>[4x]MKYVVVSGGVISGIGKGVLASSTGMLLKTLGLKVTSIKIDPYMNIDAGTMSPLEHGECFVLDDGGETDLDLGNYERYLGITLSRDHNITTGKIYSHVISRERRGDYLGKTVQIVPHLTNAIQDWIQRVSKIPVDDTGLEPDVCIIELGGTVGDIESAPFVEAL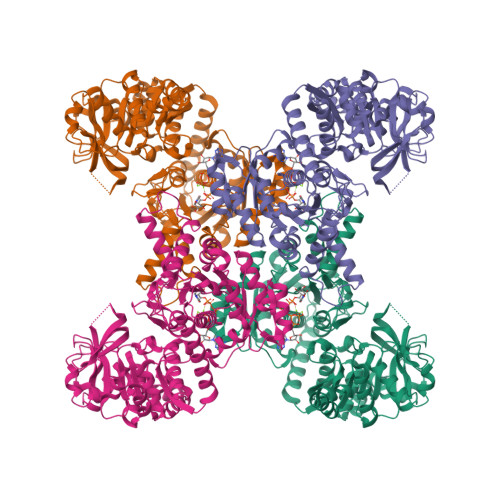RQFQFEVGRENFALIHVSLVPVIHGEQKTKPTQAAIKDLRSLGLIPDMIACRCSEELNRSTIDKIAMFCHVGPEQVVNVHDVNSTYHVPLLLLKQHMIDYLHSRLKLGEVPLTLEDKERGSQLLTNWENMTKNLDDSDDVVKIALVGKYTNLKDSYLSVTKSLEHASMKCRRQLEILWVEASNLEPETQEVDKNKFHDSWNKLSSADGILVPGGFGTRGIEGMILAAKWARESGVPFLGVCLGLQVAAIEFARNVIGRPNSSSTEFLDETLLAPEDQVVITMRLGLRPTIFQPNSEWSNIRKLYGEVNEVHERHRHRYEINPKIVNDMESRGFIFVGKDETGQRCEIFELKGHPYYVGTQYHPEYTSKVLEPSRPFWGLVAAASGTLGEVIKDINL>[4x]MTPSHPARPSRSGILVFDVNETLLDLTSLSPLFERVFGDAKVLREWFPELILYSQTLTLTGLYRPFGEIAAAVFEMVAANHQAKVTPDDIAELKTRLTSM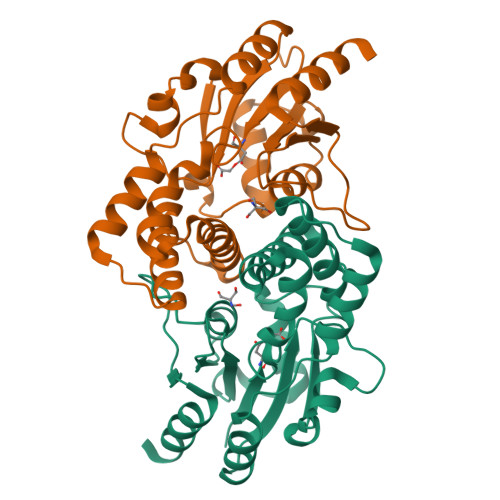PAYPDVAPALTRLQDAGFRLVTLTNSAPSPAPSPLEKAGIASFFEAHLTVHSSQRFKPHPSVYDSTAETLGAKPEELCMIACAIWDTIGAQARGWRGGFVARPHNTPLTLAEVPQPDFIGRDMGELADQLIASLTA> SMIKSYAAKEAGGELEVYEYDPGELRPQDVEVQVDYCGICHSDLSMIDNEWGFSQYPLVAGHEVIGRVVALGSAAQDKGLQVGQRVGIGWTARSCGHCDACISGNQINCEQGAVPTIMNRGGFAEKLRADWQWVIPLPENIDIESAGPLLCGGITVFKPLLMHHITATSRVGVIGIGGLGHIAIKLLHAMGCEVTAFSSNPAKEQEVLAMGADKVVNSRDPQALKALAGQFDLIINTVNVSLDWQPYFEALTYGGNFHTVGAVLTPLSVPAFTLIAGDRSVSGSATGTPYELRKLMRFAARSKVAPTTELFPMSKINDAIQHVRDGKARYRVVLKA;> MIKSYAAKEAGGELEVYEYDPGELRPQDVEVQVDYCGICHSDLSMIDNEWGFSQYPLVAGHEVIGRVVALGSAAQDKGLQVGQRVGIGWTARSCGHCDACISGNQINCEQGAVPTIMNRGGFAEKLRADWQWVIPLPENIDIESAGPLLCGGITVFKPLLMHHITATSRVGVIGIGGLGHIAIKLLHAMGCEVTAFSSNPAKEQEVLAMGADKVVNSRDPQALKALAGQFDLIINTVNVSLDWQPYFEALTYGGNFHTVGAVLTPLSVPAFTLIAGDRSVSGSATGTPYELRKLMRFAARSKVAPTTELFPMSKINDAIQHVRDGKARYRVVLKADY

Escherichia coli possess strong alcohol dehydrogenases that could contribute to producing alcohols through a designed pathway. These powerful enzymes, including YjgB, YahK, and YqhD, show nicotinamide adenine dinucleotide phosphate (NADP)-dependent activities for a variety of aldehydes. YqhD belongs to the family III metal-dependent polyol dehydrogenases, while YjgB and YahK are classified as members of the cinnamyl alcohol dehydrogenase family. As predicted from sequence alignment, the EcYjgB structure was found to belong to a typical cinnamyl alcohol dehydrogenase (CAD) family and sinapyl alcohol dehydrogenase (SAD) family, which consists of a nucleotide binding domain (NBD, residues 165–286) and a substrate-binding domain (SBD, residues 1–164 and 287–338). We observed a cleft between the SBD (substrate-binding domain) and NBD (nucleotide-binding domain) that forms the active site with a catalytic Zn2+ ion. It was found that the catalytic Zn2+ ion is coordinated by the tetrahedral combination of Cys41, His63, Glu64, and Cys152, which were well conserved.

The electron density of NADP is clearly shown in the NADP(H) binding site of the EcYjgB-NADP complex structure. We observed that His42, Ser43, Ser46, Gly179, Leu180, Ser199, Ser200, Asn201, Glu208, Ser285, Gly327, and Arg332 constitute the NADP(H) binding site. In addition, conserved Ser199 and Lys204 make it possible to specifically select the 2′ phosphate of NADP(H) as a stabilizing 2′ phosphate of the dinucleotide while using a hydrogen bond and charge-charge interaction. As it is holding the NADP, the SBD moves about 4.0 Å toward the NBD with a root-mean-square deviation (r.m.s.d.) of 1.02 Å when compared to the apo structure. It represents that NADP binding can generate the closed form, as observed in other CAD/SAD family. Meanwhile, each position of the four residues was 0.6 Å farther away from catalytic zinc in the EcYjgB-NADP complex, based on its superimposed structure with the apo form through the NBD region. During the determination of the structure comprising NADP, we found that a polyethylene glycol (PEG) fragment occupied its catalytic cavity, which was quite similar to a hexanaldehyde. Phe273′ turns toward the substrate binding site since PEG occupies the substrate-binding pocket after the conformational change upon NADP binding. Consequently, the oxygen from PEG nearby Phe273′ could form a kind of anion–π interaction that contributes to holding the ligand. Trp52 and Trp91 were shown to hold the ligand through CH-π stacking, which appeared to be a primary contributor for substrate recognition.>[2x]MEFTTGLMSLDTALNEMLSRVTPLTAQETLPLVQCFGRILASDVVSPLDVPGFDNSAMDGYAVRLADIASGQPLPVAGKSFAGQPYHGEWPAGTCIRIMTGAPVPEGCEAVVMQEQTEQMDNGVRFTAEVRSGQNIRRRGEDISAGAVVFPAGTRLTTAELPVIASLGIAEVPVIRKVRVALFSTGDQLQLPGQPLGDGQIYDTNRLAVHLMLEQLGCEVINLGIIRDDPHALRAAFIEA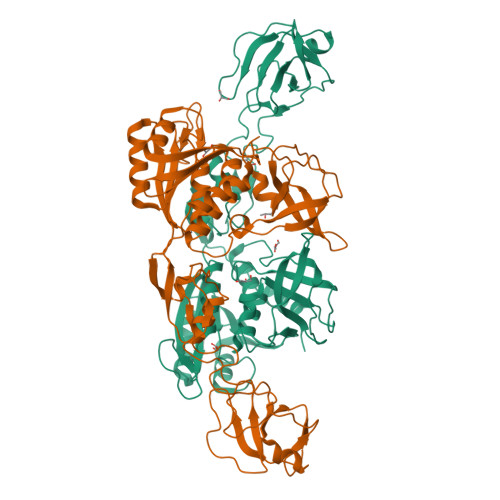DSQADVVISSGGVSVGEADYTKTILEELGEIAFWKLAIKPGKPFAFGKLSNSWFCGLPGNPVSATLTFYQLVQPLLAKLSGNTASGLPARQRVRTASRLKKTPGRLDFQRGVLQRNADGELEVTTTGHQGSHIFSSFSLGNCFIVLERDRGNVEVGEWVEVEPFNALFGGL> MNVVDISRWQFGITTVYHFIFVPLTIGLAPLIAVMQTLWVVTDNPAWYRLTKFFGKLFLINFAIGVATGIVQEFQFGMNWSEYSRFVGDVFGAPLAMEGLAAFFFESTFIGLWIFGWNRLPRLVHLACIWIV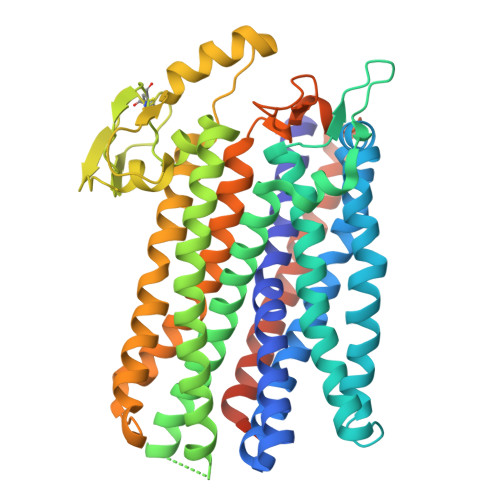AIAVNVSAFFIIAANSFMQHPVGAHYNPTTGRAELSSIVVLLTNNTAQAAFTHTVSGALLTAGTFVAAVSAWWLVRSSTTHADSDTQAMYRPATILGCWVALAATAGLLFTGDHQGKLMFQQQPMKMASAESLCDTQTDPNFSVLTVGRQNNCDSLTRVIEVPYVLPFLAEGRISGVTLQGIRDLQQEYQQRFGPNDYRPNLFVTYWSFRMMIGLMAIPVLFALIALWLTRGGQIPNQRWFSWLALLTMPAPFLANSAGWVFTEMGRQPWVVVPNPTGDQLVRLTVKAGVSDHSATVVATSLLMFTLVYAVLAVIWCWLLKRYIVEGPLEHDAEPAAHGAPRDDEVAPLSFAY> MAKVQVNNVVVLDNPSPFYNPFQFEITFECIEDLSEDLEWKIIYVGSAESEEYDQVLDSVLVGPVPAGRHMFVFQADAPNPGLIPDADAVGVTVVLITCTYRGQEFIRVGYYV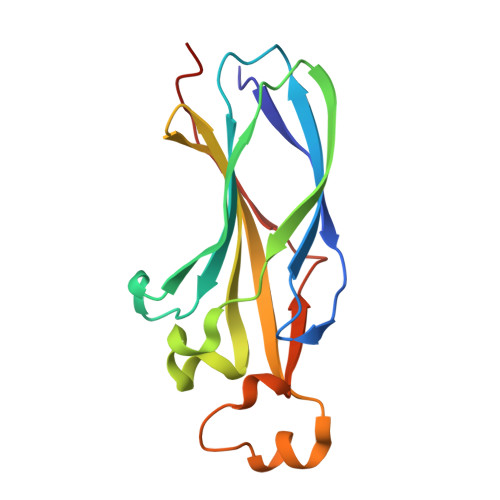NNEYTETELRENPPVKPDFSKLQRNILASNPRVTRFHINWEDN>[2x]QPSRFLLKVLAGAN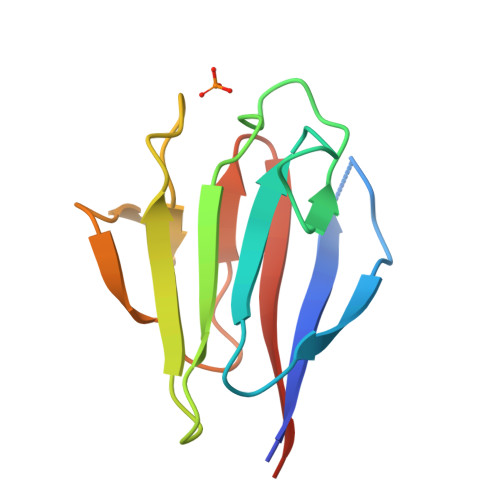IGAEFHLDSGKTYIVGSDPQVADIVLSDMSISRQHAKIIIGNDNSVLIEDLGSKNGVIVEGRKIEHQSTLSANQVVALGTTLFLLVDYAAPS>[2x]PDPMKNTCKLLVVADHRFYRYMGRGEESTTTNYLIELIDRV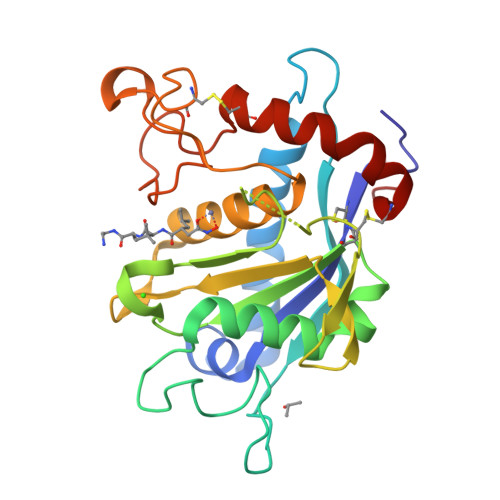DDIYRNTAWDNAGFKGYGIQIEQIRILKSPQEVKPGEKHYNMAKSYPNEEKDAWDVKMLLEQFSFDIAEEASKVCLAHLFTYQDFDMGTLGLAYGGSPRANSHGGVCPKAYYSPVGKKNIYLNSGLTSTKNYGKTILTKEADLVTTHELGHNFGAEHDPDGLAECAPNEDQGGKYVMYPIAVSGDHENNKMFSQCSKQSIYKTIESKAQECFQERS>[6x]GPAGSMKPQIRNMVEPMDPRTFVSNFNNRPILSGLDTVWLCCEVKTKDPSGPPLDAKIFQGKVYPKAKYHPEMRFLRWF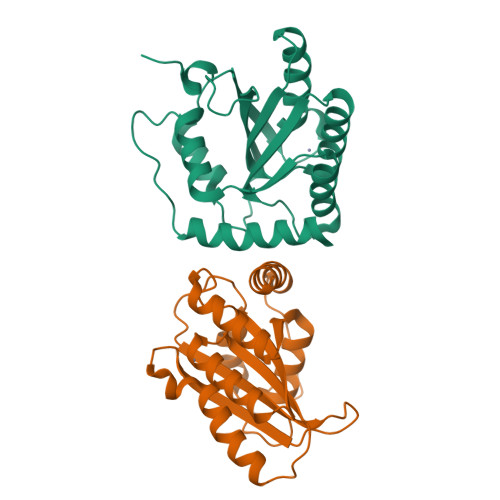HKWRQLHHDQEYKVTWYVSWSPCTRCANSVATFLAKDPKVTLTIFVARLYYFWKPDYQQALRILAEAGATMKIMNYNEFQDCWNKFVDGRGKPFKPWNNLPKHYTLLQATLGELLRH The human nucleoporin Nup98 forms fusion proteins in certain types of malignant leukaemia, is a critical component of the permeability barrier of the nuclear pore complex and is mislocalized in cytosolic deposits in Alzheimer’s disease. Key to these Nup98 activities is its large FG-repeat domain with a high number of FG motifs. The most aggregation-prone segment comprises residues 85–124 (named Nup98FG85). All four fibril types display a parallel in-register β-structure comprising short and kinked β-strands.

To gain insight into the molecular organization of cohesive FG-repeat interactions, Nup98FG85 was allowed to aggregate in pure water. EM revealed the formation of well-defined and mostly separated amyloid fibrils. Using cryo-EM, we determined the structures of four different fibril polymorphs (pm1–pm4). The least populated polymorph, pm4, was reconstructed at a resolution of 3.4 Å and contains two protofilaments related by an approximate 21 screw symmetry. The most common motif shared by the four polymorphs is a 13-residue β-turn/β-arch structure. A leucine-phenylalanine pair (L91-F92) is located at the tip of the β-turn, with both side chains pointing away from the turn. The other LF motifs in the four fibril structures show a very similar structure. In all four Nup98FG85 fibril structures, side chains stacked along the fibril axes build glutamine and asparagine ladders (top). Most of the stabilizing interactions arise where there are clusters of two to four phenylalanine rings and one or more leucine side chains. We obtained values of approximately −20 kcal mol–1 per chain for the four Nup98FG85 fibril structures.

>[11x]TGTANTLFGTASTGTSLFSSQNNAFAQNKPTGFGNFGTST> GFGCNGPWDEDDMQCHNHCKS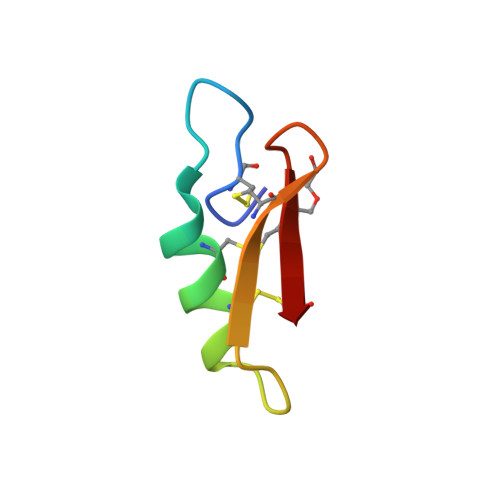IKGYKGGYCAKGGFVCKCY> EDELYRQSLEIISRYLREQATGAKDTKPMGRSGATSRKALETLRRVGDGVQRNHETAFQGMLRKLDIKNEDDVKSLSRVMIHVFSDGVTNWGRIVTLISFGAFVAKHLKTINQESCIEPLAESITD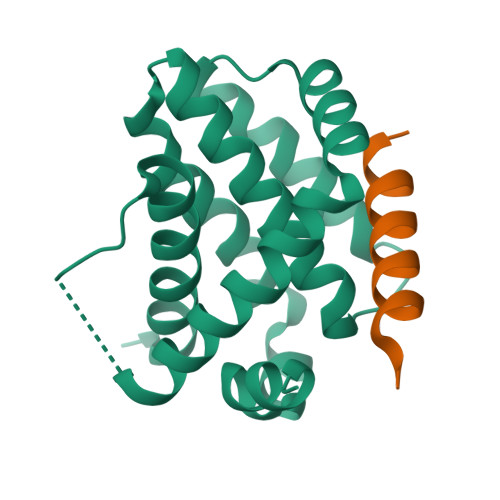VLVRTKRDWLVKQRGWDGFVEFFHVEDLEGG;> EVQIARKLQCIADQFHRLHVQ> GVEEKKSLEILLKDDRLDTEKLCTFSQRFPLPSMYRALVWKVLLGILPPHHESHAKVMMYRKEQYLDVLHALKVVRFVSDATPQAEVYLRMYQLESGKLPRSPSFPLEPDDEVFLAIAKAMEEMVEDSVDCYWITRRFVNQLNTKYRDSLPQLPKAFEQYLNLEDGRLLTHLRMCSAAPKLPYDLWFKRCFAGCLPESSLQRVWDKVVSGSCKILVFVAVEILLTFKIKVMALNSAEKITKFLENIPQDSSDAIVSKAIDLWHKH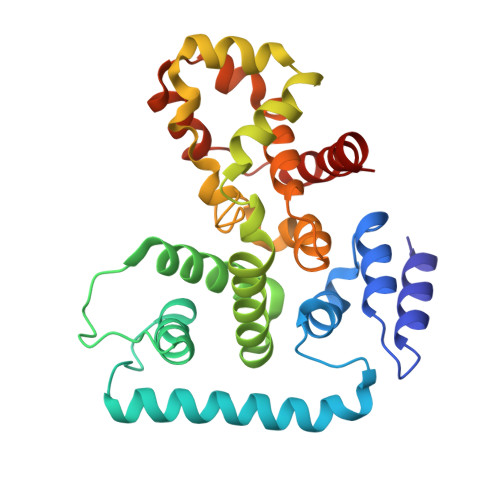CG>GMKPIKEIADQLELKDDILYPYGHYIAKIDHRFLKSLENHEDGKLILVTAVTPTPAGEGKTTTSIGLSMSLNRIGKKSIVTLREPSLGPTLGLKGGATGGGRSRVLPSDEINLHFTGDMHAVASAHNLLAAVLDSHIKHGNELKIDITRVFWKRTMDMNDRALRSIVIGLGGSANGFPREDSFIITAASEVMAILALSENMKDLKERLGKIIVALDADRKIVRISDLGIQGAMAVLLKDAINPNLVQTTEGTPALI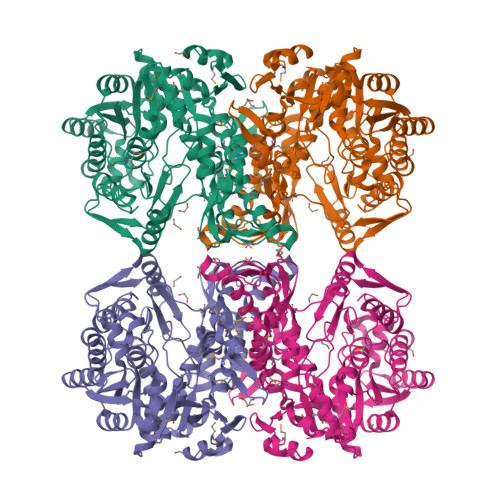HCGPFANIAHGTNSIIATKMAMKLSEYTVTEAGFGADLGAEKFIDFVSRVGGFYPNAAVLVATVRALKYHGGANLKNIHEENLEALKEGFKNLRVHVENLRKFNLPVVVALNRFSTDTEKEIAYVVKECEKLGVRVAVSEVFKKGSEGGVELAKAVAEAAKDVEPAYLYEMNDPVEKKIEILAKEIYRAGRVEFSDTAKNALKFIKKHGFDELPVIVAKTPKSISHDPSLRGAPEGYTFVVSDLFVSAGAGFVVALSGDINLMPGLPKKPNALNMDVDDSGNIVGVS[2x]> AMFLQRPKPYSDESLESFFIRVANKNGYGDVHRFLEATKRFLQDIDHNGYQTFPTDITRINPYSAKNSSSARTASFLKLAQLTFNEPPELLGLAINRTNMKYSPSTSAVVRGAEVFPRSLLRTHSIPCCPLCLRENGYASYLWH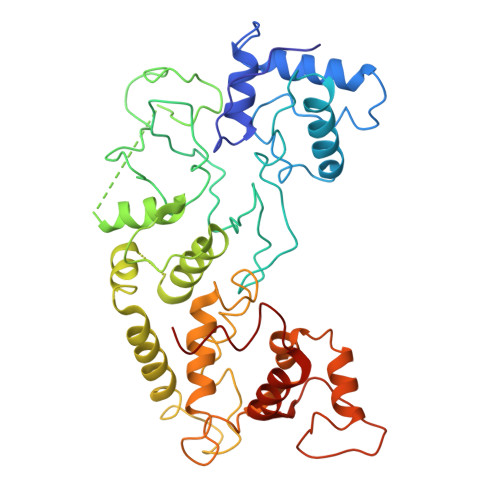FQGYEYCHSHNVPLITTCSCGKEFDYRVSEAACTVSNWLAGHESKPLPNLPKSYRWGLVHWWMGIKDDHFSFVQFFSNWPRSFHSIIEDEVEFNLEHAVVSTSELRLKDLLGRLFFGSIRLPERNLQHNIILGELLCYLENRLWQDKGLIANLKMNALEATVMLNCSLDQIASMVEQRILKPNAAAAAAAAADVTDYLFHFGDIFCLWLAEFQSDEFNRSFYVSR N-{3-[(5-cyclopropyl-2-{[3-(2-oxopyrrolidin-1-yl)phenyl]amino}pyrimidin-4-yl)amino]propyl}cyclobutanecarboxamide 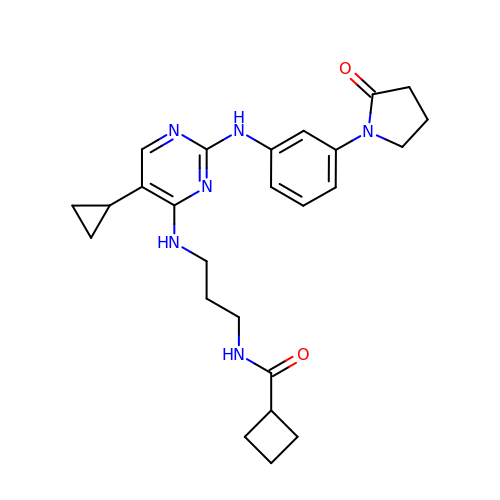| C25 H32 N6 O2 | SLUGBVRQTHMCKF-UHFFFAOYSA-N> XI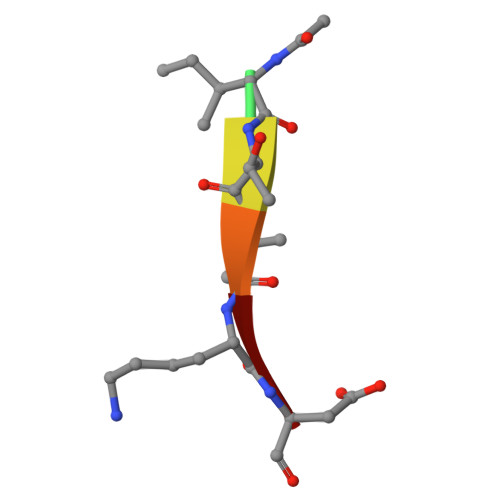TVKD> GVHVLDRPIVLFTTTGAKSGKKRYVPLMRVEENGKYAMVASKGGDPKHPSW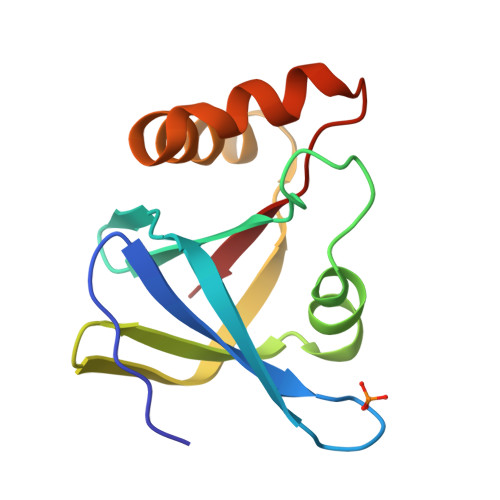YFNVKANPTVSVQDGDKVLPDRTARELEGEEREHWWKLAVEAYPPYAEYQTKTDRLIPVFIVE>MSDNDTIVAQATPPGRGGVGILRISGFKAREVAETVLGKLPKPRYADYLPFKDADGSVLDQGIALWFPGPNSFTGEDVLELQGHGGPVILDLLLKRILTIPGLRIARPGEFSERAFLNDKLDLAQAEAIADLIDASSEQAARSALNSLQGAFSARVNHLVEALTHLRIYVEAAIDFPDEEIDFLSDGKIEAQLNDVIADLDAVRAEARQGSLLREGMKVVIAGRPNAGKSSLLNALAGREAAIVTDIAGTTRDVLREHIHIDGMPLHIIDTAGLREASDEVERIGIERAWQEIEQADRVLFMVDGTTTDAVDPAEIWPEFIARLPAKLPITVVRNKADITGETLGMSEVNGHALIRLSARTGEGVDVLRNHLKQSMGFDTNMEGGFLARRRHLQALEQAAEHLQQGKAQLLGAWAGELLAEELRLAQQNLSEITGEFTSDDLLGRIFSSFCIGK[2x];>MGSSHHHHHHSSGENLYFQGMFYPDPFDVIIIGGGHAGTEAAMAAARMGQQTLLLTHNIDTLGQMSCNPAIGGIGKGHLVKEVDALGGLMAKAIDQAGIQFRILNASKGPAVRATRAQADRVLYRQAVRTALENQPNLMIFQQAVEDLIVENDRVVGAVTQMGLKFRAKAVVLTVGTFLDGKIHIGLDNYSGGRAGDPPSIPLSRRLRELPLRVGRLKTGTPPRIDARTIDFSVLAQQHGDNPMPVFSFMGNASQHPQQVPCYITHTNEKTHDVIRSNLDRSPMYAGVIEGVGPRYCPSIEDKVMRFADRNQHQIFLEPEGLTSNEIYPNGISTSLPFDVQMQIVRSMQGMENAKIVRPGYAIEYDFFDPRDLKPTLESKFIQGLFFAGQINGTTGYEEAAAQGLLAGLNAARLSADKEGWAPARSQAYLGVLVDDLCTLGTKEPYRMFTSRAEYRLMLREDNADLRLTEIGRELGLVDDERWARFNEKLENIERERQRLKSTWVTPSAEAAAEVNAHLTAPLSREASGEDLLRRPEMTYEKLTTLTPFAPALTDEQAAEQVEIQVKYEGYIARQQDEIEKQLRNENTLLPATLDYRQVSGLSNEVIAKLNDHKPASIGQASRISGVTPAAISILLVWLKKQGMLRRSA[2x]

MnmE and MnmG form a conserved protein complex responsible for the addition of a 5-carboxymethylaminomethyl (cmnm) group onto the wobble uridine of several transfer RNAs (tRNAs). Within this complex, both proteins collaborate intensively to catalyze a tRNA modification reaction that involves glycine as a substrate in addition to three different cofactors, with FAD and NADH binding to MnmG and methylenetetrahydrofolate (5,10-CH2-THF) to MnmE. MnmE is a homodimeric protein of 50–55 kDa subunits, with each protomer composed of three discernable domains: an N-terminal domain required for constitutive dimerization and binding of 5,10-CH2-THF, a helical domain and a Ras-like GTPase domain (G domain) that is inserted in the helical domain. Within the MnmEG complex, MnmG is responsible for binding the cofactors FAD and NADH, and it is also the main driver for binding of the tRNA substrate.

In the α2β2 complex, the MnmE (α2) and MnmG (β2) dimers assemble alongside each other in an elongated heterotetramer leaving one MnmE and one MnmG subunit vacant on each side of the complex. In contrast to all previously solved crystal structures that show MnmE as a symmetric homodimer in an “open” conformation with the G domains of each subunit facing but not contacting each other, the GppNHp-bound MnmE dimer (α2) within the α2β2 complex adopts a “closed” conformation, where the two G domains contact each other. However, in the α2β2 complex the MnmE dimer shows very pronounced differences in conformation between the subunit that is located at the periphery of the α2β2 complex (A subunit) and the subunit contacting MnmG (B subunit). The large conformational changes in the B subunit of MnmE in the α2β2 complex go hand in hand with a displacement of the swivel helix toward the entrance tunnel that leads to the MnmG-bound FAD. However, while previous crystal structures of MnmG from E. coli (EcMnmG), Chlorobaculum tepidum (CtMnmG), and Aquifex aeolicus (AaMnmG) present MnmG as a symmetric homodimer, the subunits (C and D) of MnmG within the α2β2 complex are not identical, due to the structuring of flexible regions in subunit C upon interaction with MnmE. Interestingly, we also observe very clear density in the EM map corresponding to a bound FAD molecule in subunit C of the MnmG dimer, while no such density is present in subunit D. Closer inspection of the structure shows that MnmE binds with its α-helical domain on top of the deep FAD-binding pocket of MnmG, thereby partially closing off this pocket. Moreover, within the complex the side chain amino group of the C-terminal lysine residue (K454) of MnmE is located within interaction distance of the C(4)=O carbonyl group of the isoalloxazine moiety of FAD. Interestingly, the distance between the amine group of K454 and the reactive N5 atom of FAD is 5.8 Å, sufficient to allow the presence of a methylene group covalently attached to K454.> VPIQKVQDDTKTLIKTIVTRINDISHTQSVSSKQKVTGLDFIPGLHPILTLSKMDQTLAVYQQILTSMPSRNVIQISNDLENLRDLLHVLAFSKSCHLPEASGLETLDSLGGVLEASGYSTEVVALSRLQ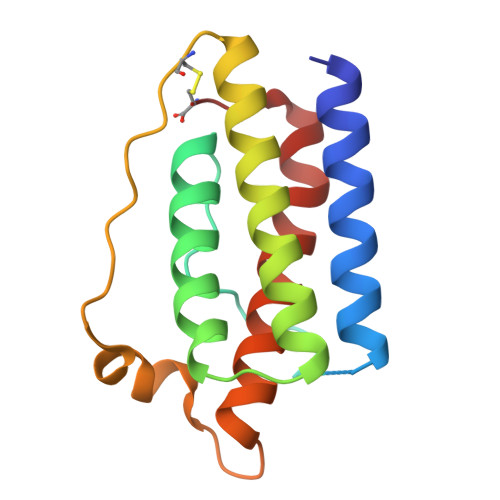GSLQDMLWQLDLSPGC> GSHMASPNGQTKPLPALKLALEYIVPCMNKHGICVVDDFLGKETGQQIGDEVRALHDTGKFTDGQLVSQKSDSSKDIRGDKITWIEGKEPGCETIGLLMSSMDDLIRHCNGKLGSYKINGRTKAMVACYPGNGTGYVRHVDNPNGDGRCVTCIYYLNKDWDAKVSGGILRIFPEGKAQFADIEPKFDRLLFFWSDRRNPHEVQPAYATRYAITVWYFDADERARAKVKYLTGEKGVRVELNK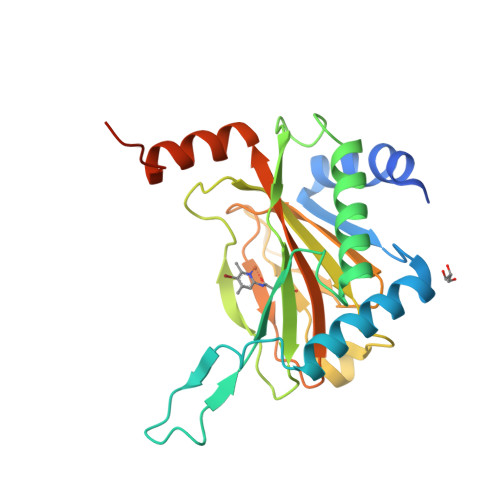PSDSVGKDVF>MIILSNEQEYVLKQVLSGVSLFYTGSAGTGKSVLLRSIIKSLRDKYPKGVAVTASTGLAACNIGGITLHSFAGFGLGQGKVENLIKKIKRNKKAFTRWRETRVLIIDEISMVDGHLLNKLNEIAKNLRRNNRPFGGIQLVACGDFYQLPPVVKKTAHDGTELDDVEVFFAFESSAWKETIQRTITLKEIFRQKGDQRFIDMLNNLRDGNVPDDTARDFCRLSRPLKCPE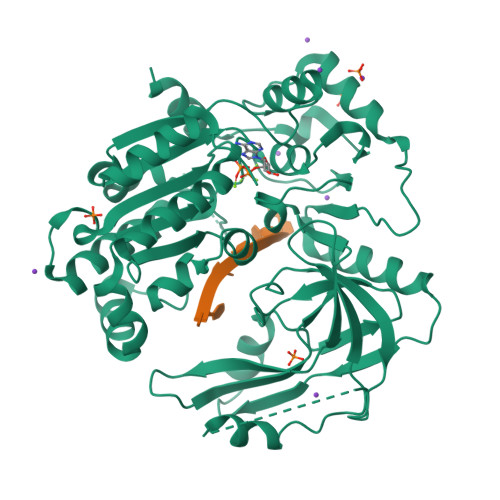GIVPSELYATRYEVDMANSRKLNTIQGDVVVYNSVDTGILPEPQKTQVLTNFLAPQVLNLKVGAQVMCIKNFDDQLVNGTLGKVIDFVDRDTYMKSESKENPSTETSDEVSGLNDYIFNDFQKPKKVVKEDAPIAEQVLFTGQLSQKVEDESESSKRKSKLKDDLMKDYKNKKYPLVKFLLPDGITFRTVVVEPEQWTTEDEDGTVLVSRIQFPLILAWSLSIHKSQGQTLSKVVVDMKKIFENGQAYVALSRAVSRAGLQVLNFNRSKVASHRKVIEFYKNLSSHEKE[2x]> MTTLLNPYFGEFGGMYVPQILMPALNQLEEAFVRAQKDPEFQAQFADLLKNYAGRPTALTKCQNITAGTRTTLYLKREDLLHGGAHTTNQVLGQALLAKRMGKSEIIAETGAGQHGVASALASALLGLKCRIYMGAKDVERQSPNVFRMRLMGAEVIPVHSGSATLKDACNEALRDWSGSYETAHYMLGTAAGPHPYPTIVREFQRMIGEETKAQILDKEGRLPDAVIACVGGGSNAIGMFADFINDTSVGLIGVEPGGHGIETG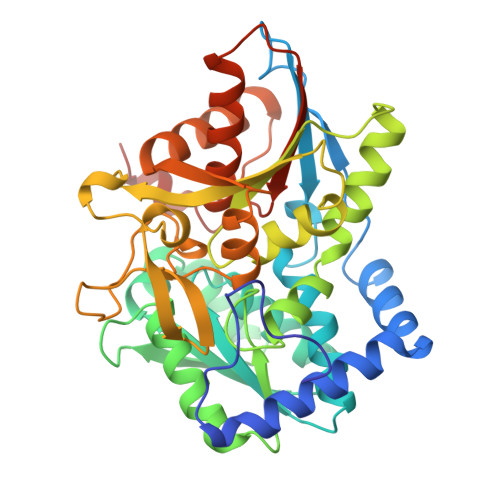EHGAPLKHGRVGIYFGMKAPMMQTADGQIEESYSISAGLDFPSVGPQHAYLNSIGRADYVSITDDEALEAFKTLCRHEGIIPALESSHALAHALKMMREQPEKEQLLVVNLSGRGDKDIFTVHDILKARGLI> GQTKAEKNGWRLGMQSYSFHLFPLTEALDKTQELGLKYIEIYPGHKLGGKWGDKVFDFNLDAQTQKEIKE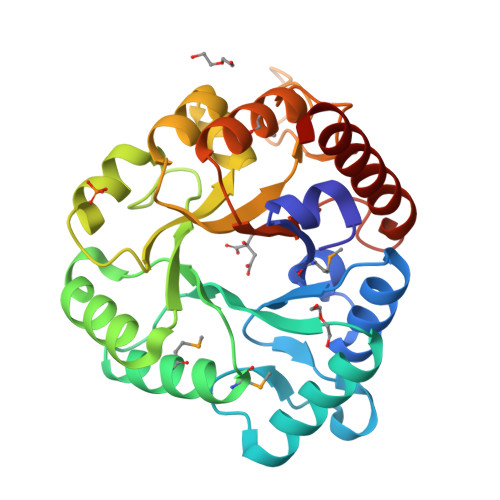LAASKGIKIVGTGVYVAEKSSDWEKMFKFAKAMDLEFITCEPALSDWDLVEKLSKQYNIKISVHNHPQPSDYWKPENLLKAISGRSQSLGSCSDVGHWRREGLNQIDCLKQLKGRIISLHFKDIAPKKAGENEQHDVIWGTGILDVKGMLKELKSQNFKGVFSIEYEYNWENSVPDIKECIQYFNKTANEIL(3~{R})-8-cyclopropyl-7-(naphthalen-1-ylmethyl)-5-oxidanylidene-2,3-dihydro-[1,3]thiazolo[3,2-a]pyridine-3-carboxylic acid | C22 H19 N O3 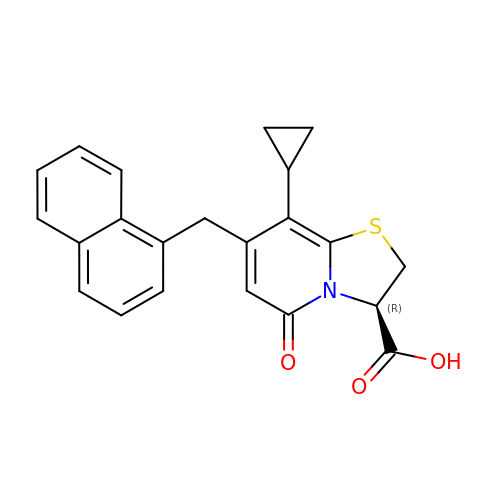S | BMDMKWJIRFLEEY-SFHVURJKSA-N>MGSDKIHHHHHHMGLFDFLKKGLQKTKETFFGRVVKLLKGKKLDDETREELEELLIQADVGVETTEYILERLEEKDGDALESLKEIILEILNFDTKLNVPPEPPFVIMVVGVNGTGKTTSCGKLAKM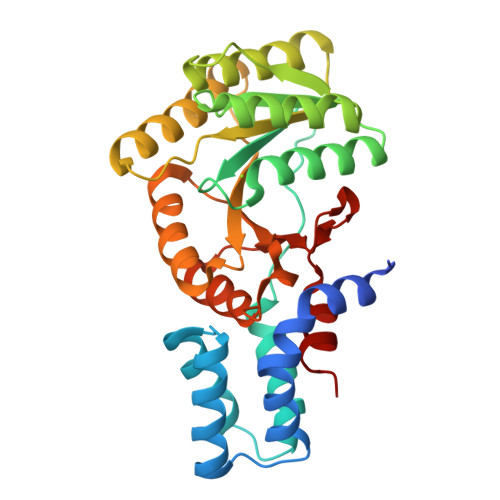FVDEGKSVVLAAADTFRAAAIEQLKIWGERVGATVISHSEGADPAAVAFDAVAHALARNKDVVIIDTAGRLHTKKNLMEELRKVHRVVKKKIPDAPHETLLVIDATTGQNGLVQAKIFKEAVNVTGIILTKLDGTAKGGITLAIARELGIPIKFIGVGEKAEDLRPFDPEAFVEVLLSE[2x]> MTIQKVHGREILDSRGNPTVEVEVTTELGVFRSAVPSGASTGIHEACELRDDDKRRYLGKGCLNAVKNVNDVLAPALVGKDELQQSTLDKLMRDLDGT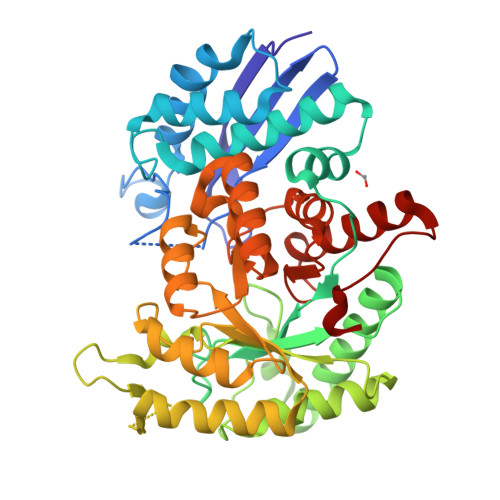PNKSKLGANAILGCSMAISKAAAARKGVPLYRYLAELAGTKEVRLPVPCFNVINGGKHAGNALPFQEFMIAPVKAGSFNEALRMGAEVYHSLKSIIKKKYGQDAVNVGDEGGFAPPITDINEPLPILMEAIEQAGHKGRFAICMDSAASETYDENKKQYNLTFKSPEATWVTAKQLAETYAKWVSEYPIVSLEDPYDQDDFDGFAGITEALKGKAQVVGDDLTVTNVSRIKTAIEKKACNSLLLKINQIGTITEAIEASKFCMSNGWSVMVSHRSGETEDTYIADLVVGLGTGQIKTGAPCRGERTAKLNQLLRIEEELGAHAKFGFPAWS>CCGGGCCCGG[2x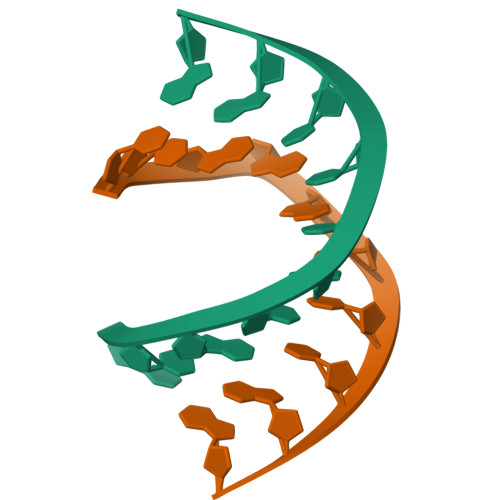]>MTLSKIKLFYNTPFNNMQNTLHFNSNEERDAYFNSKFDVHEFTSTFNYRNMKGVLRVTIDLVSDRSCFEQLMGVNYCQVQYIQSNRVEYLFVTDIQQLNDKVCELSLVPDVVMTYTQGNVLNTLNNVNVIRQHYTQTEYEQNLEQIRSNNDVLATSTMRVHAIKSELFTQLEYILTIGANLRKSFGTAEKPKFPSSSGSTHDGIYNPYDMYWFNDYESLKEVMDYLTGYPWIQQSIKNVTIIPSGFIKQESLNDHEPVNGGDLSVRKLGKQGVSNQKDFNAISLDYQSLMF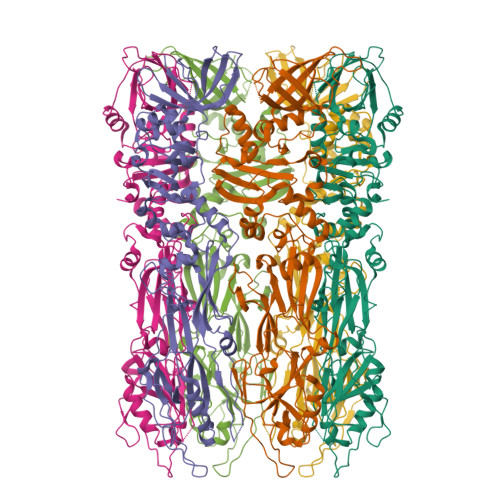TLGLNPINDKHLLRPNIVTAELTDYAGNRLPIDLSLIETNLEFDSFVTMGAKNEIKVYVKNYNARGNNVGQYIDNALTINNFDTIGFSVDSGELGKANSAYSRELSNSRQMSSRINTVLDNDASVKDRLFNAISLSGGLSIKSALSGFNNEYEHYRDQKAQFKQMDALPNAITEGHVGYAPLFKQDKFGVHLRLGRISQDELNNVKKYYNMFGYECNDYSTKLSDITSMSICNWVQFKGIWTLPNVDTGHMNMLRALFEAGVRLWHKESDMINNTVVNNVIIKSLEHHHHHH[6x]>MNHKVHHHHHHIEGRHMDEYKQVDVGKDGMVATAHPLASEIGADVLKKGGNAIDAAVAIQFALNVTEPMMSGIGGGGFMMVYDGKTKDTTIIDSRERAPAGATPDMFLDENGKAIPFSERVTKGTAVGVPGTLKGLEEALDKWGTRSMKQLITPSIKLAEKGFPIDSVLAEAISDYQEKLSRTAAKDVFLPNGEPLKEGDTLIQKDLAKTFKLIRSKG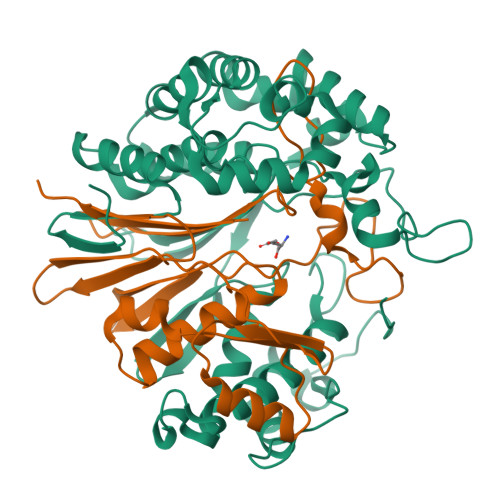TDAFYKGKFAKTLSDTVQDFGGSMTEKDLENYDITIDEPIWGDYQGYQIATTPPPSSGGIFLLQMLKILDHFNLSQYDVRSWEKYQLLAETMHLSYADRASYAGDPEFVNVPLKGLLHPDYIKERQQLINLDQVNKKPKAGDPWKYQEGSANYKQVEQPKDKVEGQ[2x];>[2x]TTHFTVADRWGNVVSYTTTIEQLFGTGIMVPDYGVILNNELTDFDAIPGGANEVQPNKRPLSSMTPTILFKDDKPVLTVGSPGGATIISSVLQTILYHIEYGMELKAAVEEPRIYTNSMSSYRYEDGVPKDVLSKLNGMGHKFGTSPVDIGNVQSISIDHENGTFKGVADSSRNGAAIGINLKRK>MSDKDSKNTPQVPEKLGLSRRGFLGASAVTGAAVAATALGGAVMTRESWAQAVKESKQKIHVGPGELDDYYGFWSGGHQGEVRVLGVPSMRELMRIPVFNVDSATGWGLTNESRHIMGDSAKFLNGDCHHPHISMTDGKYDGKYLFINDKANSRVARIRLDIMKCDKMITVPNVQAIHGLRLQKVPHTKYVFANAEFIIPHPNDGKVFDLQDENSYTMYNAIDAETMEMAFQVIVDGNLDNTDADYTGRFAAATCYNSEKAFDLGGMMRNERDWVVVFDIHAVEAAVKAGDFITLGDSKTPVLDGRKKDGKDSKFTRYVPVPKNPHGCNTSSDGKYFIAAGKLSPTCSMIAIDKLPDLFAGKLADPRDVIVGEPELGLGPLHTTFDGRGNAYTTLFIDSQVVKWNMEEAVRAYKGEKVNYIKQKLDVHYQPGHLHASLCETNEADGKWLVALSKFSKDRFLPVGPLHPENDQLIDISGDEMKLVHDGPTFAEPADCIMARRDQIKTKKIWDRNDPFFAPTVEMAKKDGINLDTDNKVIRDGNKVRVYMTSMAP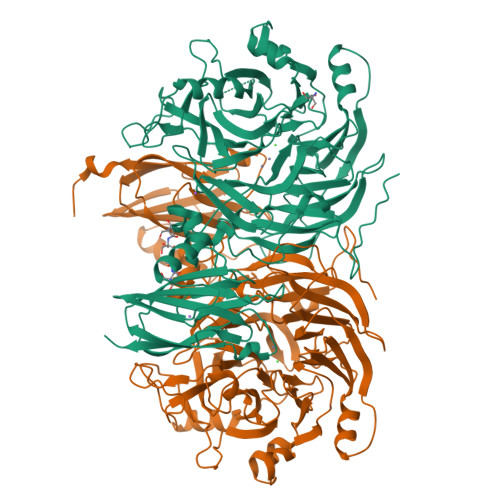AFGVQEFTVKQGDEVTVTITNIDQIEDVSHGFVVVNHGVSMEISPQQTSSITFVADKPGLHWYYCSWFCHALHMEMVGRMMVEPAWSHPQFEK[2x]> MAWPKVQPEVNIGVVGHVDHGKTTLVQAITGIWTSKHSEELKRGMTIKLGYAETNIGVCESCKKPEAYVTEPSCKSCGSDDEPKFLRRISFIDAPGHEVLMATMLSGAALMDGAILVVAANEPFPQPQTREHFVALGIIGVKNLIIVQNKVDVVSKEEALSQYRQIKQFTKGTWAENVPIIPVSALHKINIDSLIEGIEEYIKTPYRDLSQKPVMLVIRSFDVNKPGTQFNELKGGVIGGSIIQGLFKVDQEIKVLPGLRVEKQGKVSYEPIFTKISSIRFGDEEFKEAKPGGLVA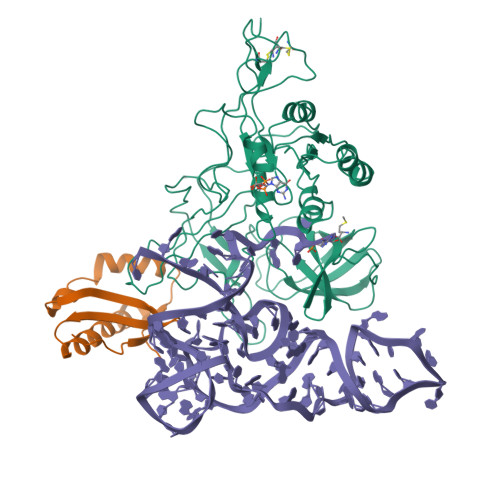IGTYLDPSLTKADNLLGSIITLADAEVPVLWNIRIKYNLLERVVGAKEMLKVDPIRAKETLMLSVGSSTTLGIVTSVKKDEIEVELRRPVAVWSNNIRTVISRQIAGRWRMIGWGLVEI;> KVKMSGLITVRTNEPLGVEKIKEVISKALENIEQDYESLLNIKIYTIGAPRYRVDVVGTNPKEASEALNQIISNLIKIGKEENVDISVV> MKIFSESHKTVFVVDHCPYMAESCRQHVEFDMLVKNRTQGIIPLAPISKSLWTCSVESSMEYCRIMYDIFPFKKLVNFIVSDSGAHVLNSWTQEDQNLQELMAALAAVGPPNPRADPECCSILHGLVAAVETLCKITEYQHEARTLLMENAERVGNRGRIICITNAKSDSHVRMLEDCVQETIHEHNKLAANSDHLMQIQKCELVLIHTYPVGEDSLVSDRSKKELSPVLTSEVHSVRAGRHLATKLNILVQQHFDLASTTITNIPMKEEQHANTSANYDVELLHHKDAHVDFLKSGDSHLGGGSREGSFKETITLKWCTPRTNNIELHYCTGAYRISPVDVNSRPSSCLTNFLLNGRSVLLEQPRKSGSKVISHMLSSHGGEIFLHVLSSSRSILEDPPSISEGCGGRVTDYRITDFGEFMRENRLTPFLDPRYKIDGSLEVPLERAKDQLEKHTRYWPMIISQTTIFNMQAVVPLASVIVKESLTEEDVLNCQKTIYNLVDMERKNDPLPISTVGTRGKGPKRDEQYRIMWNELETLVRAHINNSEKHQRVLECLMACRSKP;> MPTVVVMDVSLSMTRPVSIEGSEEYQRKHLAAHGLTMLFEHMATNYKLEFTALVVFSSLWELMVPFTRDYNTLQEALSNMDDYDKTCLESALVGVCNIVQQEWGGAIPCQVVLVTDGCLGIGRGSLRHSLATQNQRSESNRFPLPFPFPSKLYIMCMANLEELQSTDSLECLERLIDLNNGEGQIFTIDGPLCLKNVQSMFGKLIDLAYTPFHAVLKCGHLTADVQVFPRPEPFVVDEEIDPIPKVINTDLEIVGFIDIADISSPPVLSRHLVLPIALNKEGDEVGTGITDDNEDENSANQIAGKIPNFCVLLHGSLKVEGMVAIVQLGPEWHGMLYSQADSKKKSNLMMSLFEPGPEPLPWLGKMAQLGPISDAKENPYGEDDNKSPFPLQPKNKRSYAQNVTVWIKPSGLQTDVQKILRNARKLPEKTQTFYKELNRLRKAALAFGFLDLLKGVADMLERECTLLPETAHPDAAFQLTHAAQQLKLASTGTSEYAAYDQNITPLHTDFSGSSTERI;> MSDIRHSLLRRDALSAAKEVLYHLDIYFSSQLQSAPLPIVDKGPVELLEEFVFQVPKERSAQPKRLNSLQELQLLEIMCNYFQEQTKDSVRQIIFSSLFSPQGNKADDSRMSLLGKLVSMAVAVCRIPVLECAASWLQRTPVVYCVRLAKALVDDYCCLVPGSIQTLKQIFSASPRFCCQFITSVTALYDLSSDDLIPPMDLLEMIVTWIFEDPRLILITFLNTPIAANLPIGFLELTPLVGLIRWCVKAPLAYKRKKKPPLSNGHVSNKVTKDPGVGMDRDSHLLYSKLHLSVLQVLMTLQLHLTEKNLYGRLGLILFDHMVPLVEEINRLADELNPLNASQEIELSLDRLAQALQVAMASGALLCTRDDLRTLCSRLPHNNLLQLVISG;> MSAQGDCE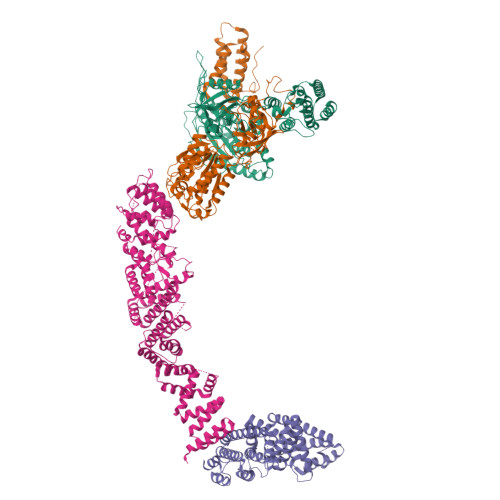FLVQRARELVPQDLWAAKAWLITARSLYPADFNIQYEMYTIERNAERTATAGRLLYDMFVNFPDQPVVWREISIITSALRNDSQDKQTQFLRSLFETLPGRVQCEMLLKVTEQCFNTLERSEMLLLLLRRFPETVVQHGVGLGEALLEAETIEEQESPVNCFRKLFVCDVLPLIINNHDVRLPANLLYKYLNKAAEFYINYVTRSTQIENQHQGAQDTSDLMSPSKRSSQKYIIEGLTEKSSQIVDPWERLFKILNVVGMRCEWQMDKGRRSYGDILHRMKDLCRYMNNFDSEAHAKYKNQVVYSTMLVFFKNAFQYVNSIQPSLFQGPNAPSQVPLVLLEDVSNVYGDVEIDRNKHIHKKRKLAEGREKTMSSDDEDCSAKGRNRHIVVNKAELANSTEVLESFKLARESWELLYSLEFLDKEFTRICLAWKTDTWLWLRIFLTDMIIYQGQYKKAIASLHHLAALQGSISQPQITGQGTLEHQRALIQLATCHFALGEYRMTCEKVLDLMCYMVLPIQDGGKSQEEPSKVKPKFRKGSDLKLLPCTSKAIMPYCLHLMLACFKLRAFTDNRDDMALGHVIVLLQQEWPRGENLFLKAVNKICQQGNFQYENFFNYVTNIDMLEEFAYLRTQEGGKIHLELLPNQGMLIKHHTVTRGITKGVKEDFRLAMERQVSRCGENLMVVLHRFCINEKILLLQTLT>[2x]METALLTLDTLAKYLQEKEVQLDIEENG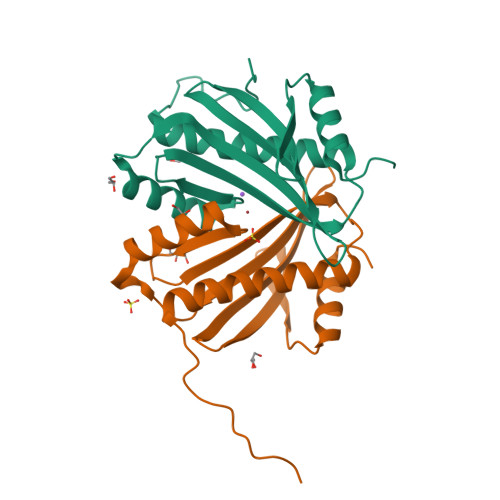GQRFIRMGWRFEMGDAAVLVSVNDGPNNTSRLEITCVTQKTYADRRAEVAMMLNDRNRERAFARSIDQEGNVWLEYVGFYPTLAEMPQETFDTLFGGVLMHFQDDYAALEGYVPQEGMQIQQPQA> GPHMEEIMQSDSKIEKMLPDGGRLVVFPNGTRKELSADGQTVKVMFFNGDVKHTMPDQRVIYYYAEAQTTHITYPDGMEVLQFPNNQTVKHFPDGRKEITFPDQTVKTLHPDGREESVLTDGTIIQLNPDGSKVIQFNTGQREIHTADFKRREYPDGTVKTVYSDG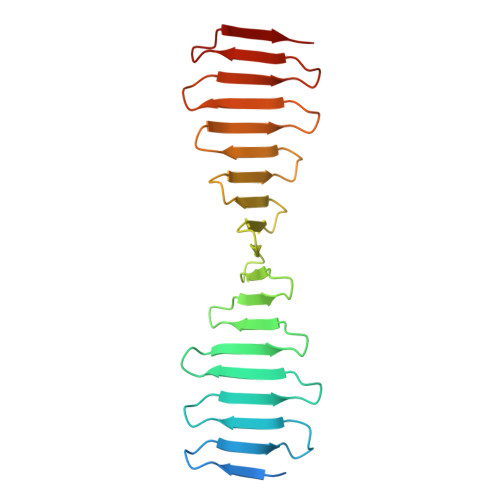RQETQYPTGRVRLKDPQGKVIMDTKA4-[(5-methyl-1,2-oxazol-3-yl)methyl]-7-[4-(1-methylpiperidin-4-yl)butyl]-2H-1,4-benzoxazin-3(4H)-one 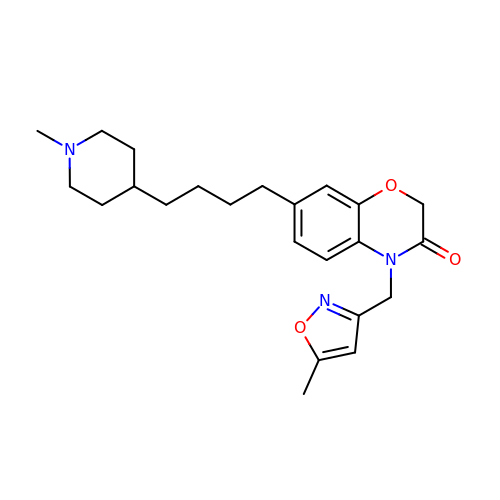| C23 H31 N3 O3 | GCGQNNSUCNJBSC-UHFFFAOYSA-N>KYVKVQDFYDQLGKYVLVAPGKFSGTVAATDLSTGWTMAWLAAWNYGDTCPIMHHMAAFPSPDPYKEFEFVVNTQGGKNLFIYGVPVTVEDPGEGMKIYRIKYDGTRMNLQRDAAEVSGLGLGVHVTITPEADGYAVGDGQKDICAEFDRETDMVRYAWAFDWDPNVKDLKRAWLDGGTMTIKRLKPTLPGGRYDLQGSKGNKIDWELVPGGELAIEDGKVSGDRPLHSVANDALVFDPRGKWAVASMRLPGVCVVFDRENQVPVAVLAGPKGTPSQFQLVKVDDDTWTVDIPEVISAGHQAGFSPDGQSFLFMNSLRQNNIMVWDSS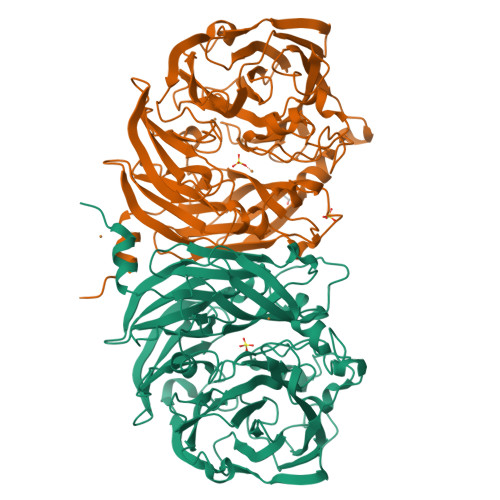NHDDPTTWEKKAVVESPDWRGAYPNTFHMVFTPDAKKIYVTMWWPSPTPNGIAVIDAVNWEVLKEVDLGPDMHTLAITYDGKFVVGTLSGYQNTASAIVVMETETDEVLGFLPSPMGHHDNVIVPRTLEDLRISRSTTT[4x]> GHMKKRVGIEALAVAVPSRYVDIEDLARARGVDPAKYTAGLGAREMAVTDPGEDTVALAATAAARLIRQQDVDPSRIGMLVVGTETGIDHSKPVASHVQGLLKLPRTMRTYDTQHACYGGTAGLMAAVEWIASGAGAGK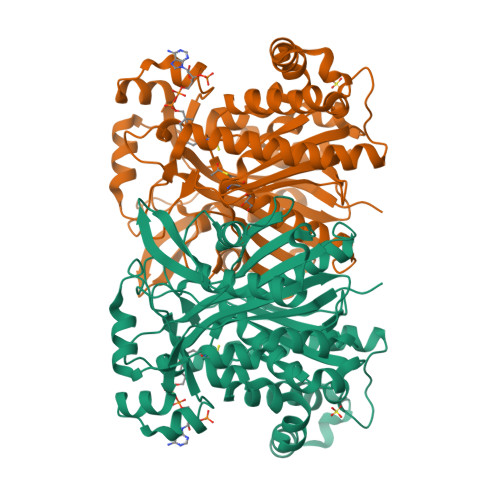VAVVVCSDIARYGLNTAGEPTQGGGAVALLVSEQPDLLAMDVGLNGVCSMDVYDFWRPVGRREALVDGHYSITCYLEALSGAYRGWREKALAAGLVRWSDALPGEQLARIAYHVPFCKMARKAHTQLRLCDLEDAADAAASTPESREAQAKSAASYDAQVATSLGLNSRIGNVYTASLYLALAGLLQHEAGALAGQRIGLLSYGSGCAAEFYSGTVGEKAAERMAKADLEAVLARRERVSIEEYERLMKLPADAPEAVAPSPGAFRLTEIRDHRRQYAEG(2R)-5-methylidene-2-{(1R)-2-oxo-1-[(phenylacetyl)amino]ethyl}-5,6-dihydro-2H-1,3-thiazine-4-carboxylic 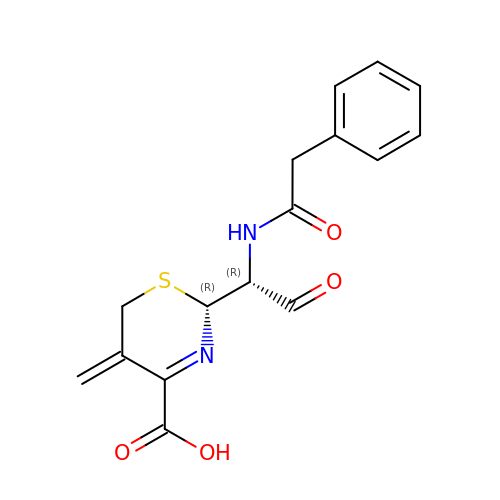acid | C16 H16 N2 O4 S | ISCTZDPSWLBTMN-IUODEOHRSA-N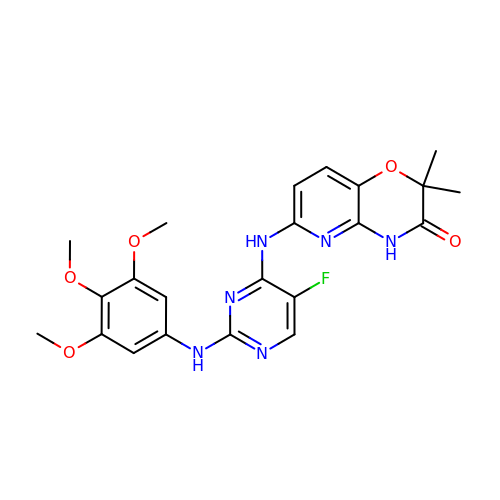6-({5-fluoro-2-[(3,4,5-trimethoxyphenyl)amino]pyrimidin-4-yl}amino)-2,2-dimethyl-2H-pyrido[3,2-b][1,4]oxazin-3(4H)-one | C22 H23 F N6 O5 | NHHQJBCNYHBUSI-UHFFFAOYSA-N> MEFGFWSALYIFVLTAFLGYELITRVPVILHTPLMSGSNFIHGVVVVGAMVVLGHAETGLEKLIGFLGVILGAANAAGGYAVTVRMLEMFERKPGQG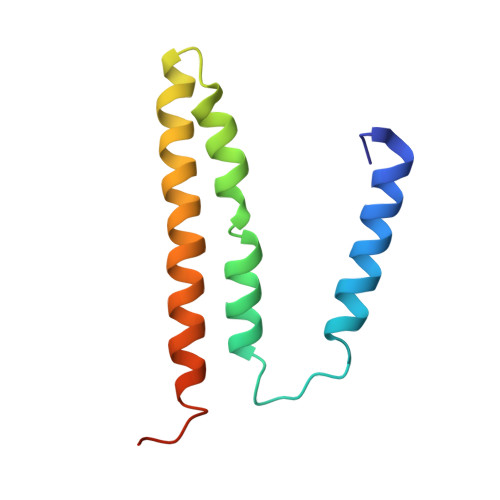GGR>SSSSGGKKCYKLENEKLFEEFLELCKMQTADHPEVVPFLYNRQQRAHSLFLASAEFCNILSRVLSRARS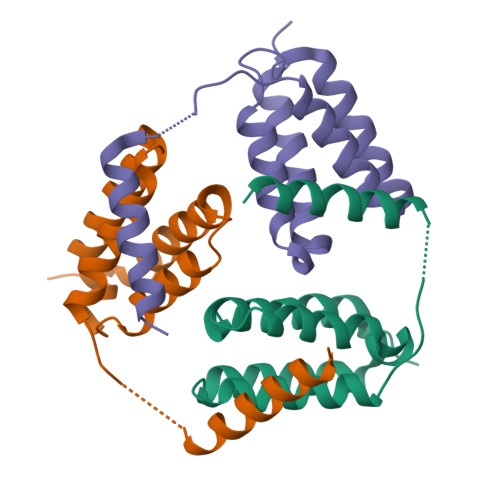RPAKLYVYINELCTVLKAHSAKKKLNNDPENRIAKKMLLEEIKANLSSDE[9x]>MAHHHHHHVDDDDKTFKMNTAQKAHYEKFINALENELKTRHIPAGAVIDMLAEINTEA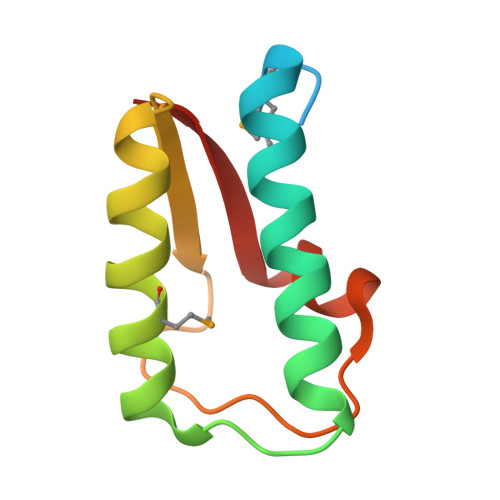LALDYQIVDKKPGTSIAQGTKAAALRKRFIPKKIK[2x]N-{3-[(2R)-1-{(2R)-2-[(1-aminoisoquinolin-6-yl)amino]-2-phenylacetyl}pyrrolidin-2-yl]-4-(propan-2-ylsulfonyl)phenyl}acetamide | C32 H35 N5 O4 S 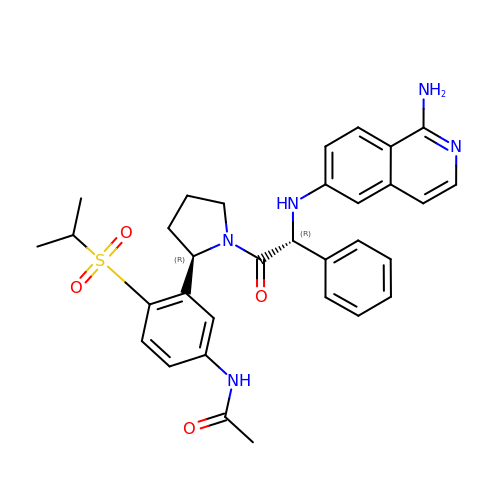| KDJVHAKXSVDSAV-PQHLKRTFSA-N> MKGMFTPG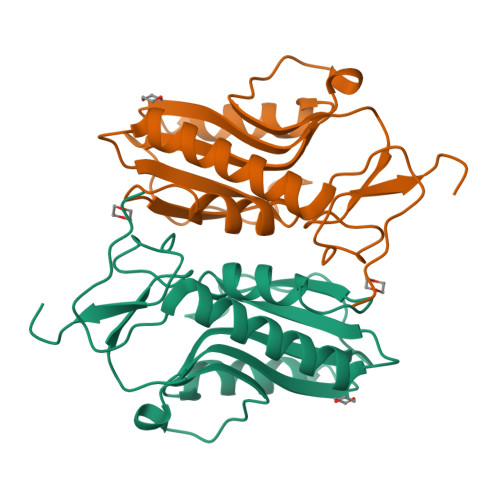NGPVQISAEAIKKRVEELGGEIARDYQGKTPHLICVLNGAFIFMADLVRAIPLPLTMDFIAISSYGNAFKSSGEVELLKDLRLPIHGRDVIVVEDIVDTGLTLSYLLDYLEARKPASVRVAALLSKPSRRQVEVPIHYLGFEIEDAYVYGYGLDRAQFDRNLPFITSIRPEEE> MPRKAREYPEEGEFVVATVKRIHNYGAFLELDEYPGKEAFMHISEVASTWVRNIRDYLKEGQKVVAKVIRVDPRKGHIDLSLRRVTQQQRKAKLQEFKRAQKAENLLRLAAEKLGKDFEAAWREVWVPLEEEWGEVYAAFEDAAKDGIEVLKGHVPDEWLPVLKEIVENYVEVPTVTIDAEFEITVPKPNGVEIIKEALIRARDRANKEK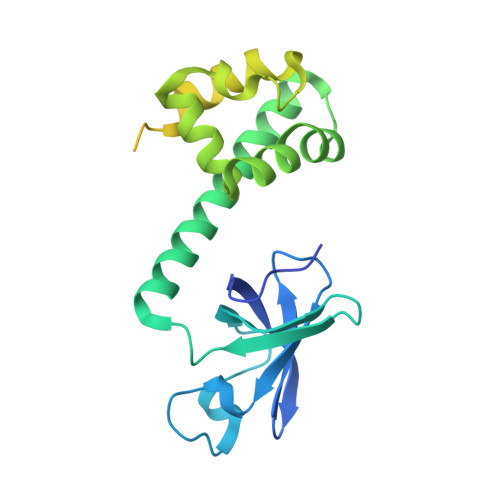DIEVKFTYQGAPRYRIDITAPDYYKAEEVLEDIAEEILRVIKQAGGEATLLRKEKRIRKVKKRKK>MFAWWGRTVYQFRYIVIGVMVALCLGGGVYGISLGNHVTQSGFYDEGSQSVAASLIGDEVYGRDRTSHVVAILTPPDDKKVTDKAWQKKVTEELDQVVKDHEDQIVGWVGWLKAPDTTDPTVSAMKTQDLRHTFISIPLQGDDDDEILKNYQVVEPELQQVNGGDIRLAGLNPLASELTGTIGEDQKRAEVAAIPLVAVVLFFVFGTVIAAALPAIIGGLAIAGALGIMRLVAEFTPVHFFAQPVVTLIGLGIAIDYGLFIVSRFREEIAEGYDTEAAVRRTVMTSGRTVVFSAVIIVASSVPLLLFPQGFLKSITYAIIASVMLAAILSITVLAAALAILGPRVDALGVTTLLKIPFLANWQFSRRIIDWFAEKTQKTKTREEVERGFWGRLVNVVMKRPIAFAAPILVVMVLLIIPLGQLSLGGISEKYLPPDNAVRQSQEQFDKLFPGFRTEPLTLVMKREDGEPITDAQIADMRAKALTVSGFTDPDNDPEKMWKERPANDSGSKDPSVRVIQNGLENRNDAAKKIDELRALQPPHGIEVFVGGTPALEQDSIHSLFDKLPLMALILIVTTTVLMFLAFGSVVLPIKAALMSALTLGSTMGILTWMFVDGHGSGLMNYTPQPLMAPMIGLIIAVIWGLSTDYEVFLVSRMVEARERGMSTAEAIRIGTATTGRLITGAALILAVVAGAFVFSDLVMMKYLAFGLLIALLLDATIIRMFLVPAVMKLLGDDCWWAPRWMKRVQEKLGLGETELPDERKRPTVRESETDQRALVGVGAHHHHHH[2x]

The mycobacterial membrane protein large 3 (MmpL3) transporter is essential and required for shuttling the lipid trehalose monomycolate (TMM), a precursor of mycolic acid (MA)-containing trehalose dimycolate (TDM) and mycolyl arabinogalactan peptidoglycan (mAGP), in Mycobacterium species, including Mycobacterium tuberculosis and Mycobacterium smegmatis. A detailed analysis suggested that MmpL3 is a TMM flippase that is absolutely essential for transporting TMMs across the cell membrane. MmpL3 consists of 12 transmembrane helices (TMs 1 to 12) and 2 periplasmic subdomains (PDs 1 and 2). Our structural data are in line with MD simulations that indicate the major conformational change of the transporter is located at the periplasmic subdomain PD2, where this movement can easily be interpreted as a rigid body rotational motion of PD2 in relation to the PD1 subdomain.

In addition to elucidating the structures of MmpL3 via cryo-EM, we crystallized the delipidated, purified MmpL3773 transporter, which contains residues 1 to 773, in the presence of trehalose 6-decanoate (T6D). T6D is an ideal ligand to mimic the TMM lipid, as it contains a trehalose moiety and is structurally similar to TMM. Crystals of MmpL3773 bound with T6D diffracted X-rays to a resolution of 3.34 Å. Surprisingly, the data indicate that each asymmetric unit of the crystal contains 2 independent MmpL3773 monomers, where the conformations (MmpL3773-T6D I and MmpL3773-T6D II) are different from each other. Interestingly, the structures of MmpL3773-T6D I and MmpL3773-T6D II are quite different both in the periplasmic and transmembrane domains. Particularly, it is observed that TM9 of MmpL3773-T6D II tilts away from the innermost surface of the cytoplasmic membrane when compared with that of MmpL3773-T6D I. Consistent with the structure of MmpL3773-PE, each MmpL3773-T6D structure is found to create 2 substrate binding sites that are situated at cavities formed by TM7-TM10 in the transmembrane region and between PD1 and PD2 of the periplasmic domain, respectively. Each binding site is occupied by a T6D molecule. One obvious distinction between these 2 structures are the exact locations of their bound T6Ds. The 2 bound T6Ds in the MmpL3-T6D II structure seemingly shift upward and move away from the surface of the membrane by 3.2 Å (at the transmembrane binding site) and 4.2 Å (at the periplasmic binding site) in comparison with the corresponding bound T6Ds in the MmpL3-T6D I structure. It appears that these 2 structures capture different transient states of substrate transport mediated by MmpL3.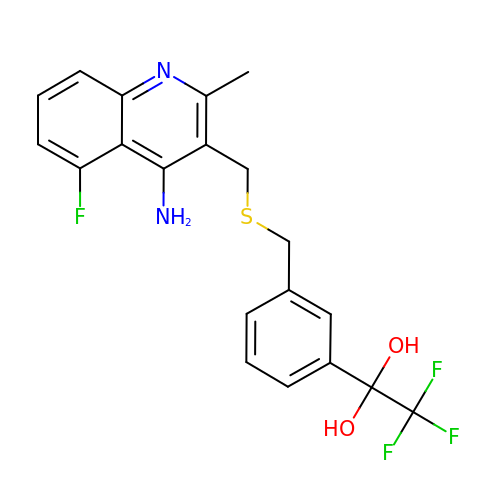1-[3-({[(4-AMINO-5-FLUORO-2-METHYLQUINOLIN-3-YL)METHYL]THIO}METHYL)PHENYL]-2,2,2-TRIFLUOROETHANE-1,1-DIOL | C20 H18 F4 N2 O2 S | GPBGHVRNVGXPNM-UHFFFAOYSA-N DIIMIDAZOLE LEXITROPSIN | C14 H20 N9 O3 | 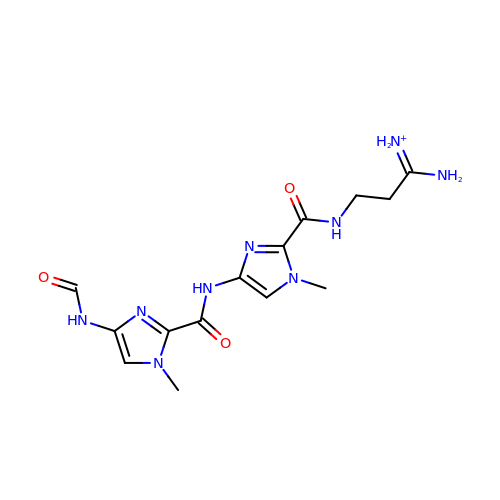WISSDOJERIUENW-UHFFFAOYSA-O>MAREESRGKRPLKIWDSWRNVRKGVVVGTFEELLVRGKDKLGVPASEPVRVVLECDGTQIEDGEYF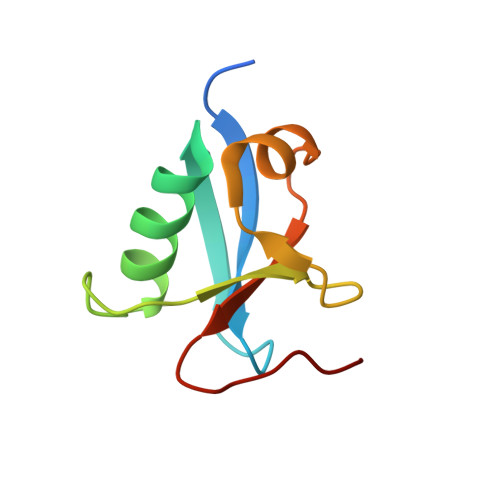RTLANNTVLLLLRQGERWLEH[4x]N-(2-amino-1H-benzimidazol-5-yl)-2-(3-chlorophenyl)acetamide 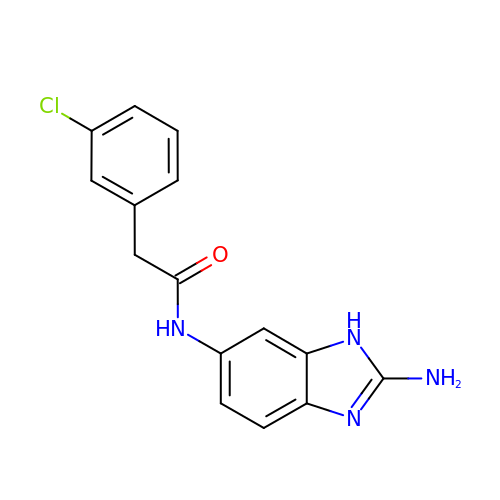| C15 H13 Cl N4 O | HFZZWILRMJMUJK-UHFFFAOYSA-N>[4x]MKNNSTVAKSTLVLLVVTCLTAFKGLAFDSISPDPIVLENGKLNINIDSKTGCFSVTEKTSGHVWKSDPWENAAGLLTLTDSKGKKQTVNISKSKKIEVSKTAKNTVSLKFIDPVFEDGSVAKGVSIATELRLDPNNAQLDVEVTEHRSGNFTLYDLRYPARAFSLKTDEDKGAAVIPQKQGVICPSYIFPMNGGRFCKWDDATYNNKSQGSLELFNNGTGLTMPWWGTYNEKSAVMGIVDVSARPHMQYNINNNGQYLFNAKGVMSPYQ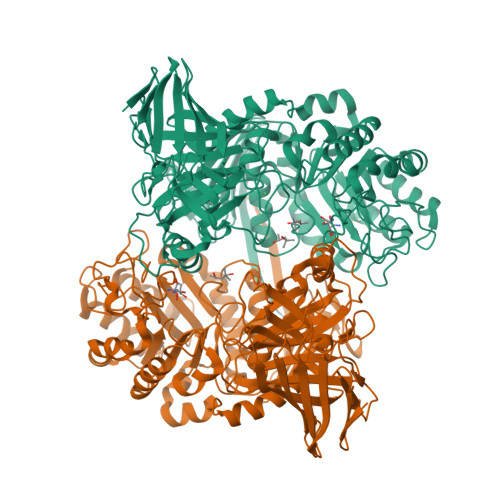RIVFLDPIWKLDQEKGKMRISYHFIPGGDYVDMAKVYQKEAKARGHFVSLQEKLKRNPNVNKLPGAIYFGIYGGYPHYVNMPGMAFTFDELKNIIKTIHDDLRVDKAFVHAWGTFSNFVPHNYPISEALGGPEKLKAAVDLAKSYGYLYSSYHAYSPMLENDPNFTTDLMQRDAEGKLMNTGSRWARVDPKFQKGLAQKNIEKEISYLGLEADITDITFAAYRENGKEGRIELAKYIDSFNLVNGTEHGQEQWIPYFDMFEGMTYLEDRPLSVISHPAPLFNLVYHEAIANFGKIQDPDNEVTANGDFRIKALRSMLFGRGTTIFFAPYEFEGMRPMIEMARDLVSPVHKETFYSELKSHEYLSADYKVQRSRFSSGTEVIANLGPVAQKIEGGISIPGYGYRIQMKDGSLKTGHFQVSLHMD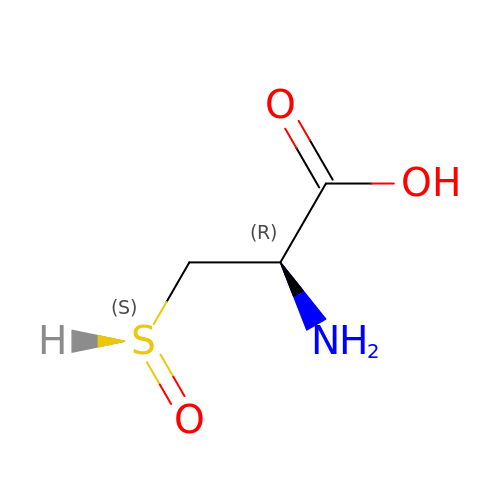S-OXY CYSTEINE | C3 H7 N O3 S | BHLMCOCHAVMHLD-REOHCLBHSA-N>[4x]MRKVKKLRLDKENTGSWRSFSLNSEGAERMATTGTPTADRGDAAATDDPAARFQVQKHSWDGLRSIIHGSRKYSGLIVNKAPHDFQFVQKTDESGPHSHRLYYLGMPYGSRENSLLYSEIPKKVRKEALLLLSWKQMLDHFQATPHHGVYSREEELLRERKRLGVFGITSYDFHSESGLF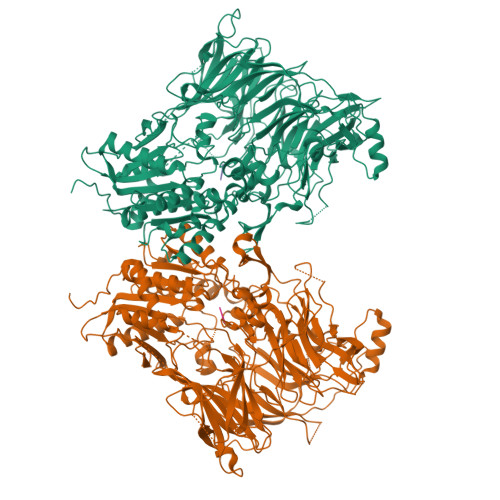LFQASNSLFHCRDGGKNGFMVSPMKPLEIKTQCSGPRMDPKICPADPAFFSFINNSDLWVANIETGEERRLTFCHQGLSNVLDDPKSAGVATFVIQEEFDRFTGYWWCPTASWEGSEGLKTLRILYEEVDESEVEVIHVPSPALEERKTDSYRYPRTGSKNPKIALKLAEFQTDSQGKIVSTQEKELVQPFSSLFPKVEYIARAGWTRDGKYAWAMFLDRPQQWLQLVLLPPALFIPSTENEEQRLASARAVPRNVQPYVVYEEVTNVWINVHDIFYPFPQSEGEDELCFLRANECKTGFCHLYKVTAVLKSQGYDWSEPFSPGEDEFKCPIKEEIALTSGEWEVLARHGSKIWVNEETKLVYFQGTKDTPLEHHLYVVSYEAAGEIVRLTTPGFSHSCSMSQNFDMFVSHYSSVSTPPCVHVYKLSGPDDDPLHKQPRFWASMMEAASCPPDYVPPEIFHFHTRSDVRLYGMIYKPHALQPGKKHPTVLFVYGGPQVQLVNNSFKGIKYLRLNTLASLGYAVVVIDGRGSCQRGLRFEGALKNQMGQVEIEDQVEGLQFVAEKYGFIDLSRVAIHGWSYGGFLSLMGLIHKPQVFKVAIAGAPVTVWMAYDTGYTERYMDVPENNQHGYEAGSVALHVEKLPNEPNRLLILHGFLDENVHFFHTNFLVSQLIRAGKPYQLQIYPNERHSIRCPESGEHYEVTLLHFLQEYLHHHHHH;>[4x]MP> MDWYEPGEDTYTLMDALEREGLEMKIVLDLGTSTGVITEQLRKRNTVVSTDLNIRALESHRGGNLVRADLLCSINQESV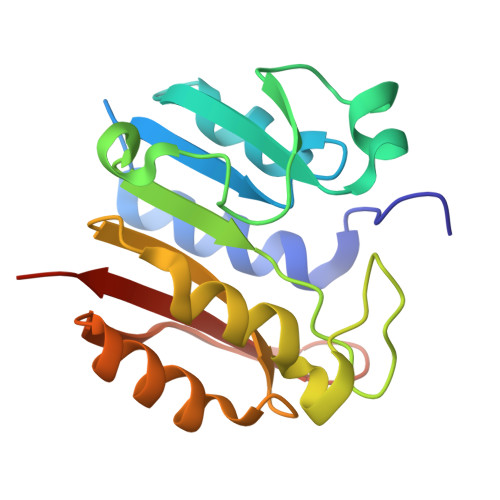DVVVFNPPYVPDTDDPIIGGGYLGREVIDRFVDAVTVGMLYLLVIEANRPKEVLARLEERGYGTRILKVRKILGETVYIIKGEKSHHHHHH>[4x]MPVFTASFQCVTLFGQPASAADAQPLLQGQRPFLHLHARRRRPCGPMLISKSPPYPASEETREWEADGQHEHTDELRETTTTMIDGIRTALRSIGEGEISISAYDTSLVALLKRLDGGDGPQFPSTIDWIVQNQLPDGSWGDASFFMMGDRIMSTLACVVALKSWNIHTDKCERGLLFIQENMWRLAHEEEDWMLVGFEIALPSLLDMAKDLDLDIPYDEPALKAIYAERERKLAKIPRDVLHSMPTTLLHSLEGMVDLDWEKLLKLRCLDGSFHCSPASTATAFQQTGDQKCFEYLDGIVKKFNGGVPCIYPLDVYERLWAVDRLTRLGISRHFTSEIEDCLDYIFRNWTPDGLAHTKNCPVKDIDDTAMGFRLLRLYGYQVDPCVLKKFEKDGKFFCLHGESNPSSVTPMYNTYRASQLKFPGDDGVLGRAEVFCRSFLQDRRGSNRMKDKWAIAKDIPGEVEYAMDYPWKASLPRIETRLYLDQYGGSGDVWIGKVLHRMTLFCNDLYLKAAKADFSNFQKECRVELNGLRRWYLRSNLEKFGGTDPQTTLMTSYFLASANIFEANRAAERLGWARVALLADAVSSHFRRIGGPKNSTSNLEELISLVPFDDAYSGSLREAWKQWLMAWTAKESSQESIEGDTAILLVRAIEIFGGRHVLTGQRPDLWEYSQLEQLTSSICCKLSRRVLAQENGESTEKVEEIDQQVDLEMQELTRRVLQGCSAINRLTRETFLHVVKSFCYVAYCSPETIDSHIDKVIFQDVIEFHHHHHH

The large superfamily of labdane-related diterpenoids is defined by the cyclization of linear geranylgeranyl pyrophosphate (GGPP), catalyzed by copalyl diphosphate synthases (CPSs) to form the basic decalin core, the copalyl diphosphates (CPPs). Here, we used X-ray crystallography and cryo-EM methods to describe different oligomeric structures of a syn-copalyl diphosphate synthase from Oryza sativa (OsCyc1), and provided a cryo-EM structure of OsCyc1D367A mutant in complex with the substrate GGPP. The structure of monomer OsCyc1 consists of an αβγ domain and a catalytic center located between the β and γ domains. OsCyc1 catalyzes GGPP to form syn-CPP, in which new bonds form between C6 and C11, as well as between C10 and C15.

To elucidate the oligomer states and the interaction mode of OsCyc1, we determined the cryo-EM structure of OsCyc1 and finally solved three OsCyc1 structures in dimer, tetramer and hexamer forms, at a resolution of 7.9 Å, 3.5 Å and 3.7 Å, respectively. The tetramer is composed of two dimers that consist of chains A/B and chains C/D. The tetramer molecules correspond to subunits A/B/C/D in the hexamer. When we analyzed the particle numbers in the cryo-EM map reconstruction, we found that the tetramer is the predominant form of OsCyc1 and is equivalent to chains A/B/C/D in the crystal structure. In the particle picking process of Cryo-EM structure determination, tetrameric assemblies are the major particles that are picked. Combined with the cryo-EM structure results, these findings imply that the major oligomeric form of OsCyc1 in solution (as used in our experiments) is tetrameric. Apart from the dimer interface, intermolecular interactions also occur between chain B and chain C, chain A and chain C, and chain B and chain D. Interactions between chain B and C are mainly located on helix α22 and involve residues S620 and D615. In chain A, β domain residues in or near α13 and α14, such as E340, R348 and Y381, interact with α domain residues of chain C in or near α19, such as R535, R539 and E543, which are identical to the interactions between chain B and chain D. Considering the results of our size exclusion chromatography and the static light scattering experiments, we hypothesized that S674A/E677A disrupts the oligomeric state of wild-type OsCyc1. Together, these results imply that the tetramer is not essential for enzyme activity in vitro.> TNTVAAYNLTWKSTNFKTILEWEPKPVNQVYTVQISTKSGDWKSKCFYTTDTECDLTDEIVKDVKQTYLARVFSYPAGNVESTGSAGEPLYENSPEFTPYL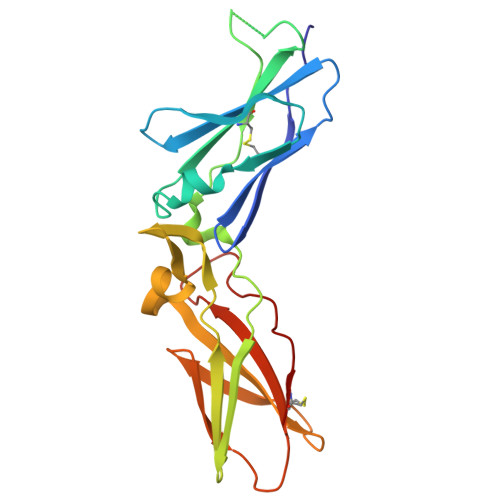ETNLGQPTIQSFEQVGTKVNVTVEDERTLVRRNNTFLSLRDVFGKDLIYTLYYWKSSSSGKKTAKTNTNEFLIDVDKGENYCFSVQAVIPSRTVNRKSTDSPVECM>[2x]IRVFDVWKKYKYYKKPQDRLKEIIFRKPFHEELWVLKGINLEIEKGEVLGIVGPNG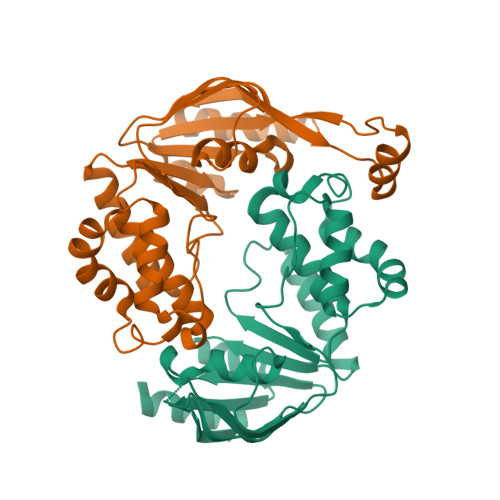AGKSTLLKVITGVTEPDKGFVERSGKVVGLLELGTGFNYELSGLENIYVNASLLGLSRREIDEKLESIIEFSELDDFINKPLKTYSSGMIMRLAFSIAIHTEPECFIIDEALAVGDAHFQQKCFRKLKEHKQKGGSIIFVSHDMNAVKILCDRAILLHKGEIIEEGSPETVTQAYYKLKLHHHHHH>XPPGPPGPPGPKGEPGPPGPPGPPGX[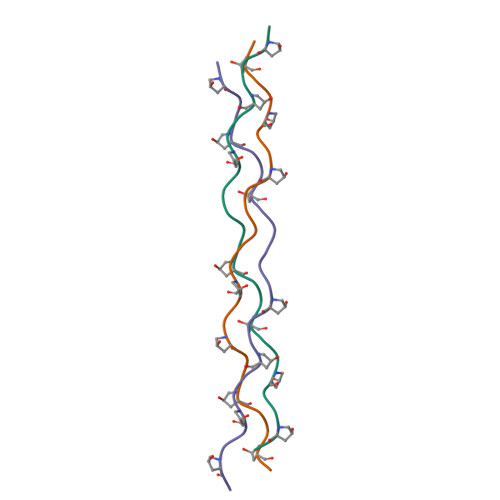6x]> 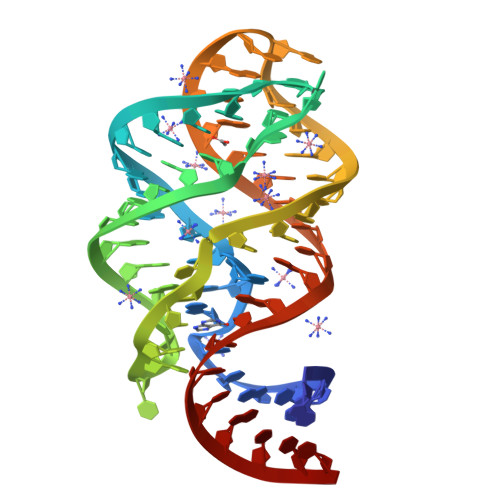GGACAUAAAAUCGCGUGGAUAUGGCACGCAAGUUUCUUCCGGGCACCGUAAAUGUCCGACUAUGUCC>AAIIGGNPYYFGNYRCSIGFSVRQGSQTGFATAGHCGSTGTRVSSPSGTVAGSYFPGRDMGWVRITSADTVTPLVNRYNGGTVTVTGSQEAATGSSVCR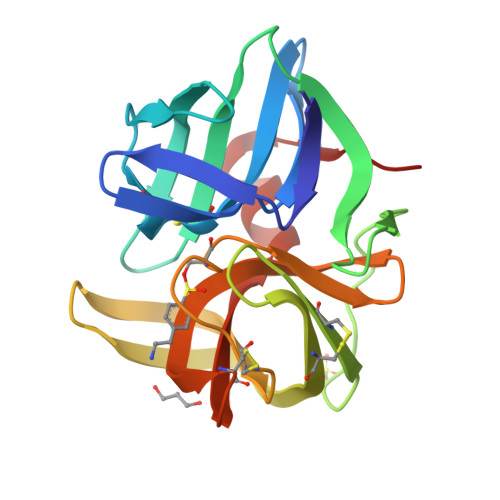SGATTGWRCGTIQSKNQTVRYAEGTVTGLTRTTACAEGGDSGGPWLTGSQAQGVTSGGTGDCRSGGITFFQPINPLLSYFGLQLVTG[2x]> G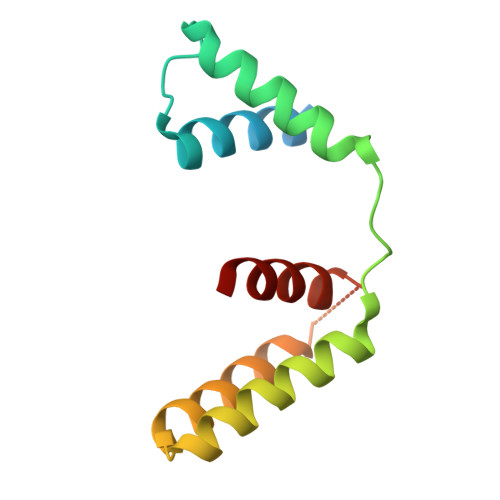PLGSMARHGPPWSRLDAQQERDVRELVRGVAGLQDEADPNFQLALNFAWSNFRFHRFLDVNSHKIEKTIEGIYEKFVIHSDLSKAASWKRLTEEFLNAPLPSIKEIKTDAHYSILSLLLCLSD>MDQKQFEKIRAVFDRSGVALTLVDMSLPEQPLVLANPPFLRMTGYTEDEILGFNCRFLQ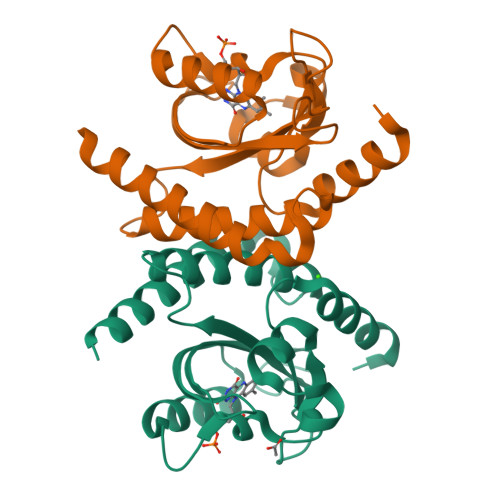RGDENAQARADIRDALKEGRELQVVLRNYRKNGEPFDNLLFLHPVGGRPDAPDYFLGSQFELGRSGNSEEAAAAGHAGALTGELARIGTVAARLEMDQRRHLAQAAAALVRAWERRG[4x]> QGFSLAQYLQEQKTIVETALDQSLVITEPVTIYEAMRYSLLAGGKRLRPILCLAACEMLGGTAAMAMNTACALEMIHTMSLIHDDLPAMDNDDLRRGKPTN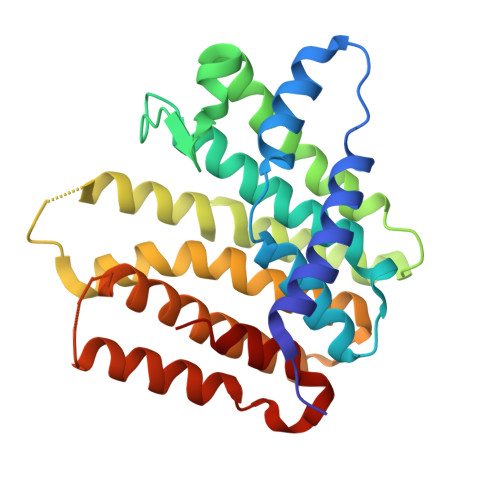HKVYGEDIAILAGDALLSYAFEYVARTPDVPAERLLQVIVRLGQAVGAEGLVGGQVVDLESETDVAVETLNFIHTHKTGALLEVCVTAGAILAGAKPEEVQLLSRYAQNIGLAFQIVDDILSLEKSQAEAQKLVAEAIASLEPYGEKANPLKALAEYI4-amino-1-[(2S,4aR,6R,7R,7aS)-2,7-dihydroxy-2-oxidotetrahydro-4H-furo[3,2-d][1,3,2]dioxaphosphinin-6-yl]pyrimidin-2(1H)-one 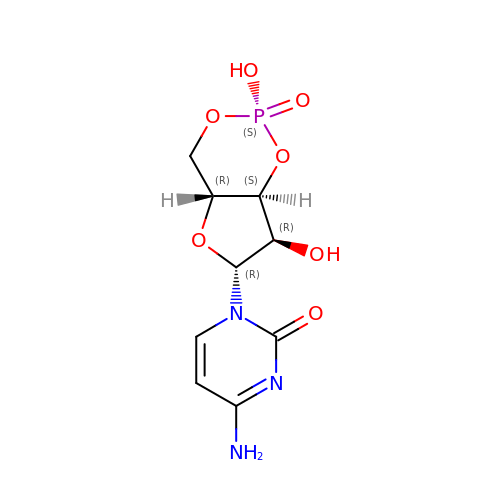| C9 H12 N3 O7 P | WCPTXJJVVDAEMW-XVFCMESISA-N>[6x]QELQELRR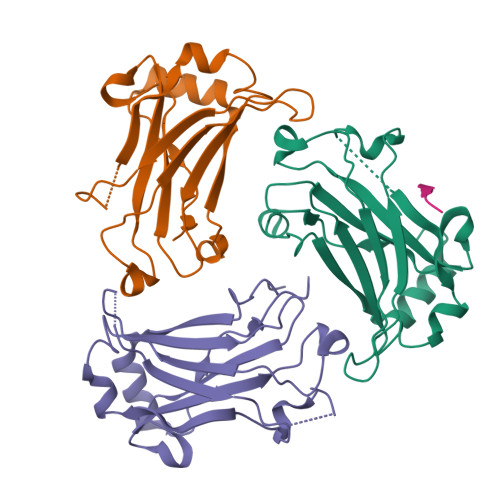ELEELSVGSDGVLIWKIGSYGRRLQEAKAKPNLECFSPAFYTHKYGYKLQVSAFLNGNGSGEGTHLSLYIRVLPGAFDNLLEWPFARRVTFSLLDQSDPGLAKPQHVTETFHPDPNWKNFQKPGTWRGSLDESSLGFGYPKFISHQDIRKRNYVRDDAVFIRAAVELPRKILS;>RLRAR[3x]Pip2(20:4/18:0) | C47 H85 O19 P3 | 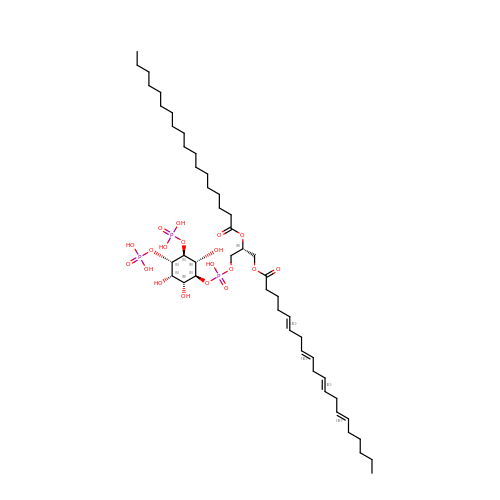WSOUXFSBLZNSFX-BSWMUMJKSA-N> ARTKQTARMSTGGKA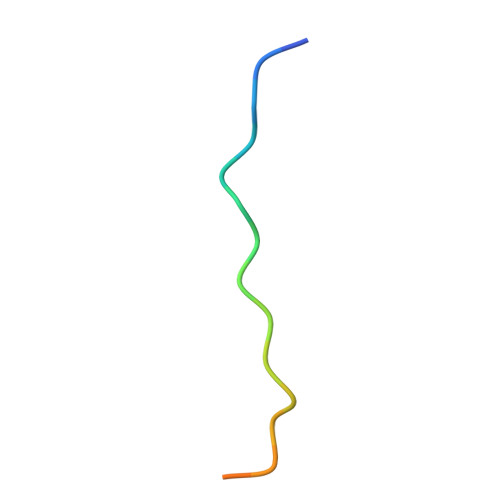PRKQ> HHHHHHMEEEAETEEQQRFSYQQRLKAAVHYTVGCLCEEVALDKEMQFSKQTIAAISELTFRQCENFAKDLEMFARHAKRTTINTEDVKLLARRSNSLLKYITDKSEE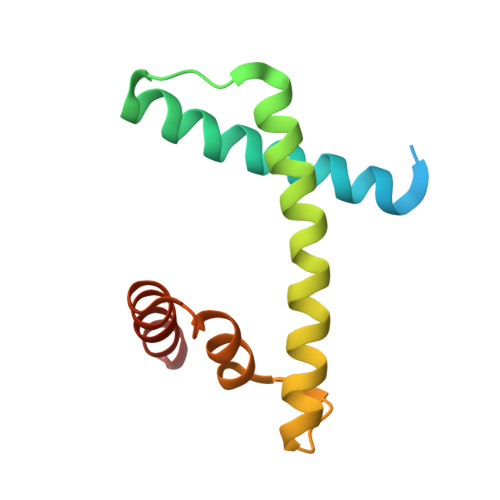IAQIN>GSEFSAMMYIQELRSGLRDMHLLSCLESLRVSLNNNPVSWVQTFGAEGLASLLDILKRLHDEKEETSGNYDSRNQHEIIRCLKAFMNNKFGIKTMLETEEGILLLVRAMDPAVPNMMIDAAKLLSALCILPQPEDMNERVLEAMTERAEMDEVERFQPLLDGLKSGTSIALKVGCLQLINALITPAEELDFRVHIRSELMRLGLHQVLQELREIENEDMKVQLCVFDEQGDEDFFDLKG[2x];>[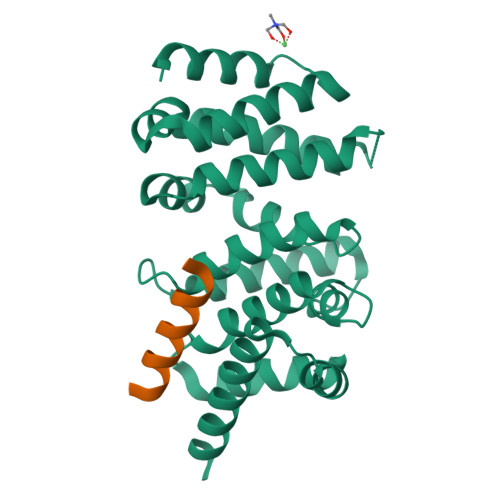2x]TPRSARLERMAQALALQAGSP> KFESKA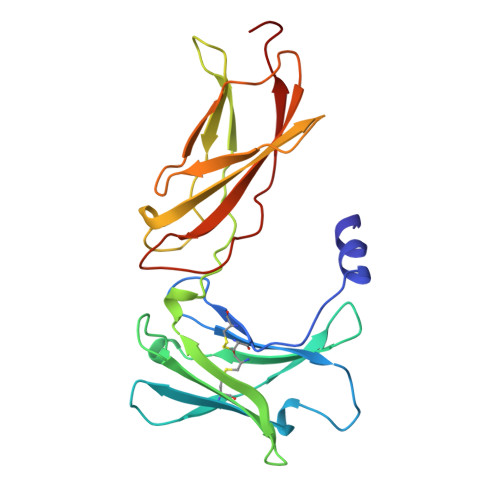ALLAARGPEELLCFTERLEDLVCFWEEAASAGVGPGNYSFSYQLEDEPWKLCRLHQAPTARGAVRFWCSLPTADTSSFVPLELRVTAASGAPRYHRVIHINEVVLLDAPVGLVARLADESGHVVLRWLPPPETPMTSHIRYEVDVSAGNGAGSVQRVEILEGRTECVLSNLRGRTRYTFAVRARMAEPSFGGFWSAWSEPVSLLTPSDL>MTERT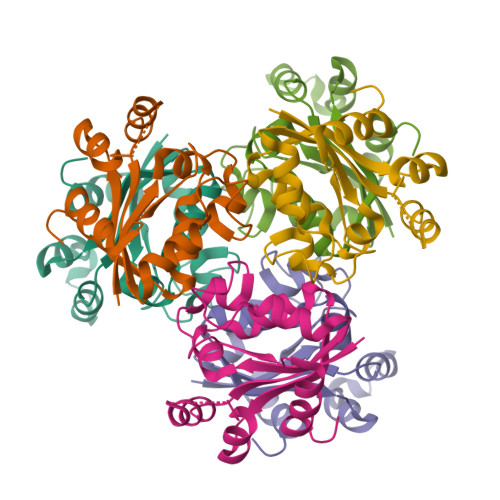LVLIKPDGIERQLIGEIISRIERKGLTIAALQLRTVSAELASQHYAEHEGKPFFGSLLEFITSGPVVAAIVEGTRAIAAVRQLAGGTNPVQAAAPGTIRGDFALETQFNLVHGSDSAESAQREIALWFPGA[2x]>MHRPEAEKWLRRFERAPDARARLVCLPHAGGSASFFFPLAKALAPAVEVLAVQYPGRQDRRHEPPVDSIGGLTNRLLEVLRPFGDRPLALFGHSMGAIIGYELALRMPEAGLPAPVHL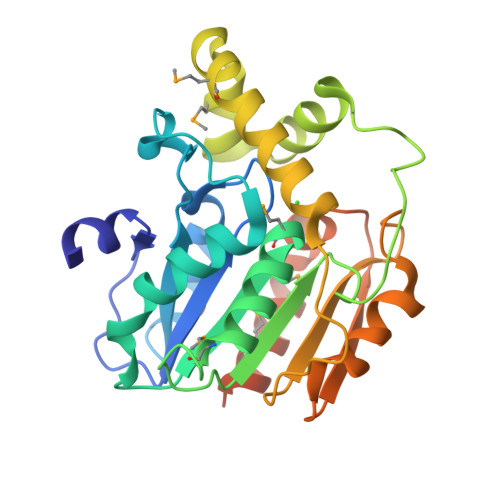FASGRRAPSRYRDDDVRGASDERLVAELRKLGGSDAAMLADPELLAMVLPAIRSDYRAVETYRHEPGRRVDCPVTVFTGDHDPRVSVGEARAWEEHTTGPADLRVLPGGHFFLVDQAAPMIATMTEKLAGPALTGSTGGNSLEHHHHHH[2x]>MWSLKSNSTALAVALNGIVALGQTITVNPSTTYQTIDGFGFSEAFGFGAPIASASASIQTQVTNYLFSTTTGAGLTILRNRIAAGSGSIEPNAPSGPNAQPTYTWDGNDAGQVWWSKQARAKGVKYIYADAWSAPAFMKTNDNVANGGYLCGTTGETCSSGDWRQAYANYLVQYIKDYANEGITIDFVGWLNEPDYSPNYDSMLITSGTQAASFIPTLYNTIKSAGLSTGIACCDPFGWSDAVTWTAQLASAGATQYLARITSHWYASKGTSPINTSLRVWETEYADLDDAFTTTWYSSGAANEGLTWANLIW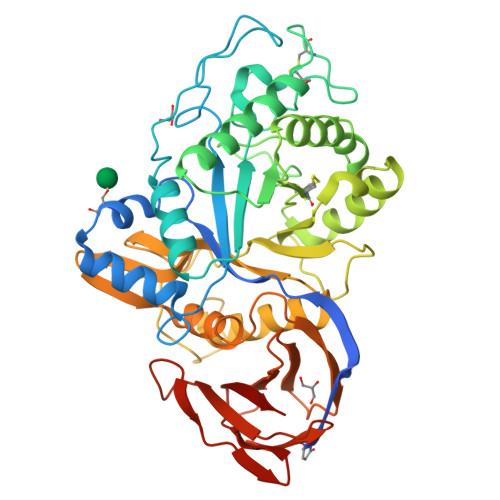QGVVEADLSAFLYWIGAQSNSNAAGLVTLNGSTVQASGTLWAFAMFSRFIRPDAVRISTSGSPSNVNVGAFKNADGSIVVVAINNNGNSETISLSGITASKVSAYYMDSAVSSPSTFSATLNGGTVGGSLPARSMVTFVITT[2x]>[2x]KKKEEKGKNIQVVVRCRPFNLAERKASAHSIVECDPVRKEVSVRTGGLADKSSRKTYTFDMVFGASTKQIDVYRSVVCPILDEVIMGYNCTIFAYGQTGTGKTFTMEGERSPNEEYTWEEDPLAGIIPRTLHQIFEKLTDNGTEFSV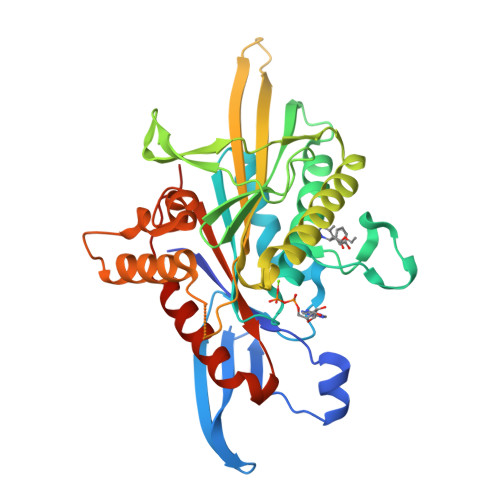KVSLLEIYNEELFDLLNPSSDVSERLQMFDDPRNKRGVIIKGLEEITVHNKDEVYQILEKGAAKRTTAATLMNAYSSRSHSVFSVTIHMKETTIDGEELVKIGKLNLVDLAGSENIGRSGAVDKRAREAGNINQSLLTLGRVITALVERTPHVPYRESKLTRILQDSLGGRTRTSIIATISPASLNLEETLSTLEYAHRAKNILNKPEVNQK>[2x]HMASQKVKEPTVSNADWSKPYRPFRIAGNLYYIGTYDLACYLITTKQGNIIVNTGLAASALQIKNNIKALGFKLTDTKILLTTQAHYDHLGAMAEIKKITGAKLMADEGDATVMADGGSSDYAFGGHGSMFEPIIADRLLHDKDTIQLGDTKLVMLHHPGHTKGSCSFLFDTKDEQRSYRILIANMPTIVIEKKFSEVSSYPGIAKDYAYTLQAMKNLSFDIWVASHASQFSMHSKHKPGDGYNPKSFMDRKGYDESLDKLQKEYEKHLNEN

In this study, we report the phenotypic, kinetic and structural analysis of a metallo-β-lactamase isolated by metagenomics from an uncultured bacterium from Alaskan soils. LRA-12 is a class B3, di-zinc dependent metallo-β-lactamase with highest amino acid identity to the Elizabethkingia meningoseptica GOB enzymes. Results show that LRA-12 exhibits a broad spectrum profile, since penicillins, cephalosporins, cephamycins and even carbapenems were hydrolyzed, with kcat/Km values ranging from 0.16 to 1.75 μM-1.s-1. In this sense, both LRA-12 and GOB enzymes present the highest carbapenemase activity among class B3 MBLs.

Metagenomic LRA-12 crystallized in space group P 1 21 1, and crystals diffracted at a final resolution of 2.1 Å. The refined structure consists in two monomers per asymmetric unit. The overall structure of LRA-12 conserves the main structural features of a class B β-lactamase, showing an αβ/βα sandwich in which α-helices are exposed to the solvent and surround a compact core of β-sheets. Interestingly, a cobalt ion was modeled between the two monomers of LRA-12 in the asymmetric unit, bound to Glu140-Oε and His175-Nε2 in a tetrahedral coordination. This cobalt, present in the crystallization buffers, could help in the crystallization process by stabilizing intermolecular interactions, as previously suggested. The catalytic cavity has a tridimensional geometry of a shallow cleft having 150–170 Å3, similar to what was reported for GOB-18 (150–200 Å3). The metal-binding site 1 is defined by Gln116, His118, and His196 (site QHH), which is uniquely found in this enzyme and in GOB β-lactamases; zinc-binding site 2 is constituted by Asp120, His121, and His263 (site DHH). Both Zn(II) ions adopt a distorted squared pyramidal molecular geometry, in which three water molecules, along with the aforementioned conserved residues, participate in the metal-coordination. In LRA-12, a water molecule occupies the position of Ser221 lateral chain in FEZ-1/BJP-1, forcing the side chain of Met221 to point outwards from the active site, which enables a displacement of the β11-α5 loop (containing Met221) that carries it, thus increasing the size of the cavity; compared to FEZ-1, BJP-1, and L1, the Cα of residue at 221 is displaced 2.70, 2.72 and 3.06 Å, respectively.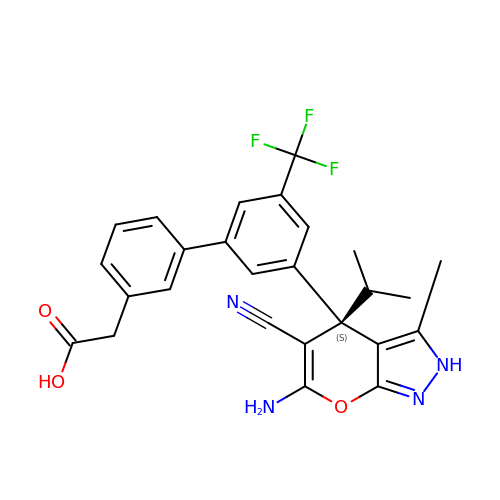2-[3-[3-[(4~{S})-6-azanyl-5-cyano-3-methyl-4-propan-2-yl-2~{H}-pyrano[2,3-c]pyrazol-4-yl]-5-(trifluoromethyl)phenyl]phenyl]ethanoic acid | C26 H23 F3 N4 O3 | DBCDVNKPJCGLLK-VWLOTQADSA-N>[2x]NNEIIPGKLKQRSIKAEGDGIVGE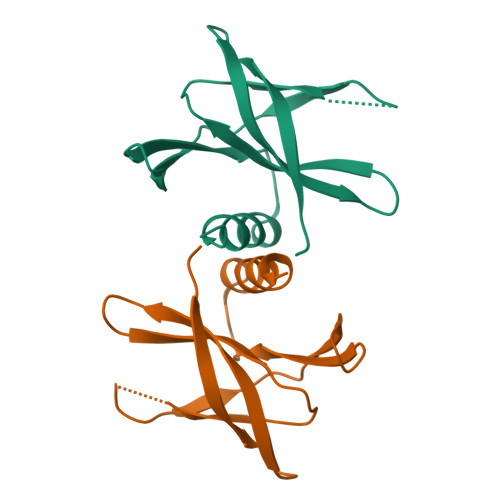GKALYNNEGGRTFMYAFISDKPDLRVVKWEFDGGCNTIELEPPRKFLVDSPNGAQIKYLYFVRNLNTLRRGAVLGYIGATVRLQHHHHHH> XMNTPKEEFQDWPIVRIAAHLPDLIVYGHFSPERPFMDYFDGVLMFVDISGFTAMTEKFSSAMYMDRGAEQLVEILNYHISAIVEKVLIFGGDILKFAGDALLALWRVERKQLKNIITVVIKCSLEIHGLFETQEWEEGLDIRVKIGLAAGHISMLVFGDETHSHFLVIGQAVDDVRLAQNMAQMNDVILSPNCWQLCDRSMIEIESVPDQRAVKVNFLKPPPNFNFDEFFTKCTTFMHYYPSGEHKNLLRLACTLKPDPELEMSLQKYVMESILKQIDNKQLQGYLSELRPVTIVFVNLMFEDQDKAEEIGPAIQDAYMHITSVLKIFQGQINKVFMFDKGCSFLCVFGFPGEKVPDELTHALECAMDIFDFCSQVHKIQTVSIGVASGIVFCGIVGHTVRHEYTVIGQKVNLAARMMMYYPGIVTCDSVTYNGSNLPAYFFKELPKKVMKGVADSGPLYQYWGRTEKV

In mammals, bicarbonate regulates the concentration of the prototypical second messenger 3′,5′cyclic adenosine monophosphate (cAMP) via the stimulation of soluble adenylate cyclases (EC 4.6.1.1).[2–4] cAMP is solely produced by adenylate or adenylyl cyclases (AC), and its intracellular levels are tightly regulated. Mammalian cells express two different types of adenylate cyclases: the well-known transmembrane ACs (tmAC) and the more recently discovered soluble adenylate cyclase (solAC). Soluble AC (solAC) is found in the cytosol, is structurally and biochemically distinct from the tmAC enzyme family, and is synergistically regulated by calcium and bicarbonate ions. Here, we describe the first crystal structures of a mammalian solAC, and the application of fragment-based drug discovery methods to identify small-molecule inhibitors of the human enzyme.

The next round of synthesis focused on molecules capable of forming a hydrogen bond with the side chain of Arg 176; this was an attractive design idea because the side chain was easily accessible and sits at the mouth of the ATP pocket. A number of heterocycles were then synthesized that could retain this hydrogen bond whilst improving the π-stacking with Phe 336. This culminated in the discovery of the novel lead compound 8 (IC50=0.36 μm). The designed molecule induces a movement of the side chain of Asp 99 to form an additional long hydrogen bond with the benzimidazole of compound 8. The molecule also forms a hydrogen bond with the flexible side chain of Arg 176, although the geometry is not ideal. The inhibitors were discovered by fragment-based drug discovery and occupy both the newly identified allosteric bicarbonate site of the protein as well as the ATP pocket.>MEHHHHHHNKDLKGLYAALLVPFDENGQVNEQGLKQIAQNAIETEELDGLYVNGSSGENFLLNTEQKKQVFKVAKEAVGDKVKLIAQVGSLDLNEAIELGKYATELGYDALSAVTPFYYPFTFEEIRDYYFDIIEATQNNMIIYAIPDLTGVNISIEQFSELFNHEKIVGVKYTAPNFFLLERIRKAFPDKLILSGCDEMLVQATISGVDGAIGSTYNVN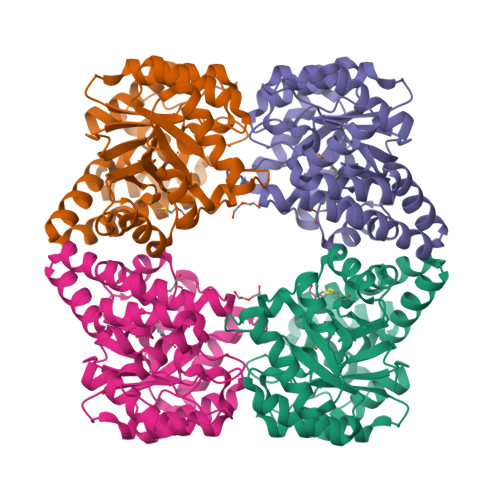GRRARKIFDLARQGQIQEAYQLQHDSNDIIETVLSMGIYPTLKEILRHRGIDAGLPKRPFKPFNEAHRQTLDQLIAKYDL[4x]> MHQHSTAALDTALAYHRAWTGRDFDTAMRHVAGGIVCHA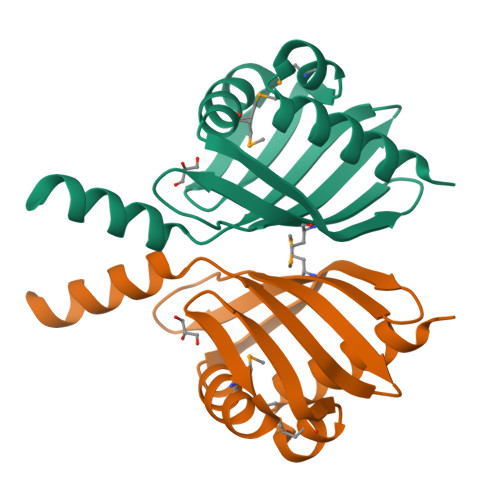PAGRIDGADAFRAFMEPFSRILVGSAVLSAFGDATTALLMYDTETVPVPHAPAAEHLTVHDGRITQLRIIFDRTPFEQARTARDEGKL>GSHMEKLAKNKVISIDAGRKYFTLNQLKRIVDKASELGYSDVHLLLGNDGLRFLLDDMTITANGKTYASDDVKKAIIEGTKAYYDDPNGTALTQAEVTELIEYAKSKDIGLIPAINSPGHMDAMLVAMEKLGIKNPQAHFDKVSKTTMDLKNEEAMNFVKALIGKYMDFFAGKTKIFNFGTDEYANDATSAQGWYYLKWYQLYGKFAEYANTLAAMAKERGLQPMAFNDGFYYEDKDDVQFDKDVLISYWSKGWWGYNLASPQYLASKGYKFLNTNGDWYYILGQKPEDGGGFLKKAIENTGKTPFNQLASTKYPEVDLPTVGSMLSIWADRPSA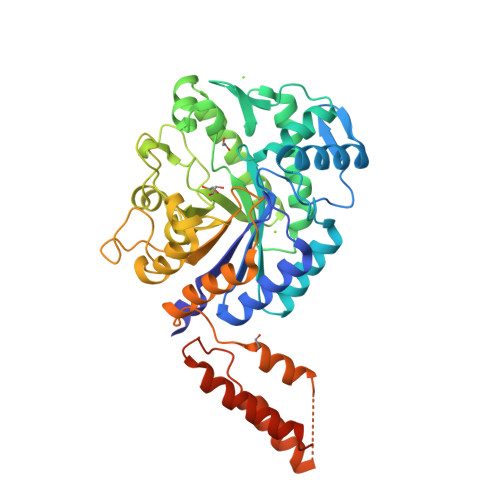EYKEEEIFELMTAFADHNKDYFRANYNALREELAKIPTNLEGYSKESLEALDAAKTALNYNLNRNKQAELDTLVANLKAALQGLKPAVTHSGSLDENEVAANVETRP[4x]>MER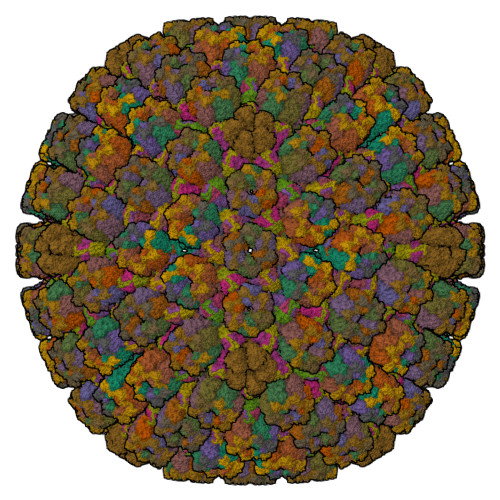PAILPSGQILSNIEVHSHRALFDIFKRFRSDDNNLYGAEFDALLGTYCSTLSLVRFLELGLSVACVCTKFPELSYVAEGTIQFEVQQPMIARDGPHPADQPVHNYMIKRLDRRSLNAAFSIAVEALGLISGENLDGTHISSAMRLRAIQQLARNVQAVLDSFERGTADQMLRVLMEKAPPLSLLAPFTLYEGRLADRVACAALVSELKRRVRDDTFFLTKHERNKDAVLDRLSDLVNCTAPSVAVARMTHADTQGRPVDGVLVTTAGVRQRLLHHVLTLADTHADVPVTYGEMVIANTNLVTALVMGKAVSNMDDVARYLLGGEPAPDDGKPVGSARVRADLVVVGDRLVFLEALEKRVYQATQVPYPLVGNLDVTFVMPLGVFKPAADRYARHAGSFAPTPGLPDPRTHPPRAVHFFNKDGVPCHVTFEHAMGTLCHPSFLDVDATLAALRQEPAEVQCAFGAYVADARPDALVGLMQRFLEEWPGMMPVRPRWAAPAAADQLLAPGNADLRLELHPAFDFFVAPEVDVPGPFAVPQVMGQVRAMPRIINGNIPLALCPVDFRDARGFELSVDRHRLAPATVAAVRGAFRDANYPMVFYIIEAVIHGSERTFCALARLVAQCIQSYWRNTHNAAFVNNFYMVMYINTYLGNGELPEDCAAVYKDLLEHVHALRRLIGEFTLPGDPLGNQPQEELNHALADATLLPPLIWDCDPILYRDGLAERLPELRVNGAHFQHILWVEMAQVNFRNVGGGLVHNRPVRNENQPLHPHHDAEWSVLSKIYYYAVVPAFSRGNCCTMGVRYDRVYQLVQTMVVPETDEEVGTDDPRHPLHPRNLVPNSLNVLFHNACVAVDADAMLILQETVTNMAERTTPLLASVAPDAGMATVATRDMRTHDGSLHHGLLMMAYQPNDATLLEGAFFYPAPVNALFACADHLGAMRDVGAEVRAAAQHVPCVPHFLGANYYATVRQPVAQHAAQSRADENTLSYALMAGYFKMSPVAFTHQLRRQLHPGFALTVVRQDRFATENVLFAEKASESYFMGQMQVARTESGGGLHLQLTQPRANVDLGVGFTAAYAAAALRAPVTDMGNLPQNLFATRGAPPMLDADADDYLRRTVNAGNRLAPVPVFGQMLPQVPAGLARGQQSVCEFIATPVSVDLAYFRRACNPRGRAAGEVHGEEGLMFDHSHADPAHPHRATANPWASQRHSYADRLYNGQYNMSGPAYSPCFKFFTPAEAVAKSRGLARLIADTGAAASPTSNGEYQFKRPVGAGELVEDPCALFQEAYPPLCASDSALLRTPLGAEEHFAQYLIRDESPLKGCFQHASA[16x];>[10x]MEVDIALPTLSPGDLSALQRCEGRVVFLETLRRHATLREVALPCGGDVLAAMAAYRRRFAAVITRVTPHRMLATPLGVGGRGQSLVLQNTGPFDLTNGDHVCLVPPLLGDECLRLTSANLELRFPMTLPLAQARELTARVVARAAETLRGGAPARGADVVFSNGRRYQLPPPHRDNAEAATRSLVLNMIFLLNEGAVILLSLIPNLLTLGAQDGYANAVIQLGSATRELGQLVRQPPPPLPQDHARRFCVFEALEAWIASASRLGDTLGTRPVARVCIFDGPPTVPPGEKAAVVEV;>[10x]MSVQIGNGLLMVVAPGTLTVGSARARLIRQVTLADFCEPQAERPGLVVLALRHPADLAGAAYAATPPGKNHRDLEEAWLALDEGGRGLGGDGIRASVVSLNFLVAAAENADDALRAHVTTNYRDRRTAARLERFATVLRAMIRSHVFPHRALHVLGGLLGHVTQDRLASVTCVARGDQEAARTNDMAARRSQVHVPACALMDVDRELRLGGDDGLRFAYLVFVYTQRHRREALRVHVAVSRLPELGDALSFLLAGTRVDNAIHGTDEADAPAAPAAAAAFPAYLFNDPRSARCPTGRLNTPAAEALPVWAPDMRGRATRNSCMYAAYVRLGTVERVVRRAERCGSVDLPLAHMERFTWDVGAWEECFF;>MSFDPNNPRTITAQTLEGALPVDILLRLNRATGLQMDAAEAHAIVEDARRTLFIGTSLALVNLRRAHDKHLVERQPMFATSDYSSWARPTVGLKRTFCPRPPP[15x]>MFPARLSLAVLFSVSPALAYFSGLGLGSERSIFRRDLNSTGDESNSTQWPAPLANGGKSWASAFKKAKATVTEMTVEELANITSGVIGLCSGVTGAVTRLGIPEFCLQDGPIGPRGVHGSSQFPAGLTVAATWDRTLMYARARGMGQEFHDQGVHLALAPVTGGPLGRTPLNGRGWEGTFADPYACGEASYLSVKGLTDAGVATVSKHWIAYEQETSRNLYIDIDGVSQADIQLPISSNVDDLTMHELYMWSFAEAVRAGTNHIMCSYNRINNTHSCSNAKGLNQLLKTELNFQGGVVSDWGGQWDSVPAAENGLDVAMPGKGFLGALGDFWGATLVELINNGTVSEDLVRDKAVRILTGYYYLGQDTNPPPPFVYNTIGAPTLNATSGYRNVRKPGTAELIKEIGSASVTLLKNTGSLPLKHPQRIAVLGNDATYNVLGPNACGLANSACDIDNLNGTLTTGGGSGSALSPYTITPLEALQKRAIEDNAEIAAVVANSNTTTGAEDAIAALLPDADVTFVFLNRYSEEGADAPDFSLGGDGDNLMDLAVTYSSNVVVVIHTTGVVDIEKWADNPNVTAILVAYLPGQEAGNSLVPVLYGDVAPSGKLPWTWGKSIDDYVPNGVVYTDAYSPQSNFTEGVFIDYRWFDKMGITPRYEFGFGLSYTTFTYSNLIVDHGRWAKDYSSVMETAEPFAEWDGTNSLYDVIFTVFATITNTGNLTGSEVAQLYISIPGDNQPVRQLRGFDK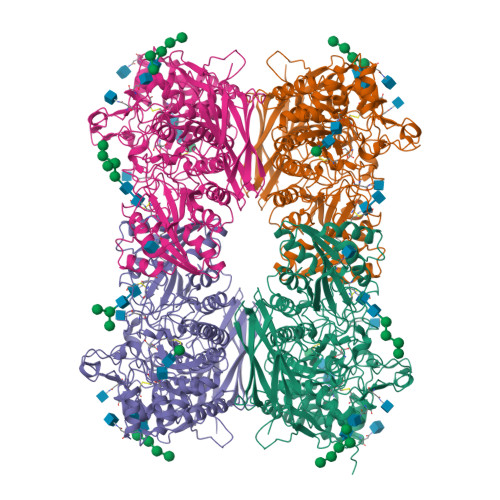IKDLPVGDSAVVTFPIRRKDVSSWSVVDQLWYVPNGDFLISVGGSSRDLPLNTTWTPHHHHHH[4x]As a sirtuin (SIR2) family protein, defense-associated sirtuin2 (DSR2) has been demonstrated to participate in bacterial anti-phage resistance via depleting nicotinamide adenine dinucleotide (NAD+) of infected cells, which can be activated by tail tube protein (TTP) and inhibited by DSR anti-defense 1 (DSAD1) of diverse phages. To defend phage invasion, Bacillus subtilis utilizes DSR2 proteins to sense and recognize phage SPR tail tube protein (TTP), then unleashes NADase activity of its SIR2 domain to deplete the cell of NAD+ and abort phage propagation during infection. Each DSR2 protomer contains three domains, an N-terminal SIR2 domain (SIR2, residues 1 to 297), a middle connector domain (MID, residues 297 to 627), and a C-terminal sensor domain (CTD, residues 627 to 1005). Structural analyses and biochemical studies reveal that DSR2 forms a tetramer with a SIR2 central core and two distinct conformations.

The determined cryo-EM structure of the DSR2-TTP complex contains DSR2A/open, DSR2B/closed, and SIR2 domains of DSR2C (DSR2C-SIR2) and DSR2D (DSR2D-SIR2), and one TTP monomer bound only to DSR2B/closed, instead of DSR2A/open. In the complex structure, owing to the remarkable flexibility of domain 2, only TTP domain 1 with residues 1 to 73 and 189 to 263 was determined. Domain 1 encompasses strands β1 to β7, which make extensive interactions with DSR2closed with a buried area of ~2900 Å2. Notably, loop 1 inserts into the CTD and loop 3 extends across the CTD to penetrate even to the MID, indicating that these two loops may play key roles in TTP binding and activation on DSR2 NADase activity. The binding pocket on CTD of DSR2B/closed widens to accommodate TTP with only a small switch of its helix α42. However, the bound TTP makes contact with the adjacent DSR2A/open, forming a hydrogen bond and a salt bridge with the α30-α31 loop of DSR2A CTD. Notably, this interaction drags the loop of DSR2A/open toward TTP with a distance of 8 Å. This dragged position is almost the one of DSR2B/closed, implying a transition state of DSR2A conformational change triggered by TTP from an open state to a closed state. The combination of TTP acts like a key, allosterically causing the MID and SIR2 domain of both protomers to undergo profound conformational changes with complicated translocation of its secondary structure elements, though the conformational changes that happened on DSR2B and DSR2A are quite different. Thus, combining with in vitro NADase hydrolysis analyses, this conformational change with a large distortion of the SIR2 domain tetramer induced by TTP is suggested to play an important role on triggering the NADase activity of DSR2.

>MVKVDLESKRYGEKLKEVFLMLDNNVVECIKEITESSRNGKLVFFVGAGVSTLSDYPQWWRLVDKYHEELYGSPKKGNYSSDEYLRIPQIFYNVKGEMAFDGILKDFFQVDKPTNPIHDKILAMNPAHVITTNYDNLIDTACWKRGKYFSVISAEEDVANATSSRYLLKVAGDFRKGFKGENVVLKEDDYLNYDQNYPLISNLMKTIIATHTIVFIGYGLGDYNINMLLNWVRKLQKDSFHKPFFIRTDPSPIENETLIYYENKGLRIIDAASLIDSNEYDYLERYSAVMDLLIESQENKFITKDDEVIDYIYGKISPLFALQYIRKIDLKHVFEYDYHFEVNGTVVRHKNKGFGYMERFFELKESCDERSKLSKKQYERFNALFNFFEKNGVICMAKDAGTLNTSIEINSLAYHGKYDVMKKFIEEQSVSIEDDYKKAFFLACLGRWEESYDLYSNIILNSIDESNGCVYYLSQINRYRIYQSITQAVTQFNGLGLLTFGRHYKPFTDEFLARIEREMTNFNIDDLFNGMPFEFQKKYKILEFLSDNQFLYDDTVKLFELTNKVRSEMSEGSYSFGMSSDIVVLLRLYDNLRFLYENCLWSVSFHEFHQYIRNSMSLLIEKAEYERTRDIDELGFSFFGKKSGFFMEYYDFVNISRHFKIDDIKNLERSCSIDKIRFGEQEKIEEYLVGIAEEITKQFSANGMNVVFYTQFISEAKAALYFAKYVKLSEEGLGKIVKALLFYFPERDLDIGKRYVWLERLTKCNELPKSIISIIDDFLVLQAEKHIDQNYSEVSSNGLYSRDYGALIKHFEKNFISKRLSEITLCLTQDKQKQIDFLFKLLPLLSTNAKSHLLSFKSVENINDLMNGIRIGLIDEFTPEHEELIIEYLETRKVNYIVEKEKGIQTFSSNDYMSTFGIWYFLEEINNSKMEEFIGMDDQYDFFVDPENFDYKKFIPSWLKNYNDKLLGKIAGNKHMKHHVIEVLKERVKNSNDKRYLEILMNYFI[4x];> MKTVIQDTADVYFKRKSDGKLVFTAEAQTASFSQAISEEKLRGGIGNKPLYILKSEKEINLTVKNAFFDLEWLAMTQGETIQEETKVKVFDREHGLIVDDTNKVTLKGKPVSDVTFYNKKGLTYKIAVSTDGTYTIPTAFAAAKDKLTAVYQIEKVGRRLAIKASKFSERYEVEYRTIAYNPDTEEVYSDIYIQFPNVSPSGEFEMSLENGNALAPEIKFEALADTDTDEMAVVIEASRDENTAAPVEDTTGSTQSSDLGGTTE Nalpha-[(2S)-2-benzyl-3-(tert-butylsulfonyl)propanoyl]-N-[(1S,2R,3S)-1-(cyclohexylmethyl)-3-cyclopropyl-2,3-dihydroxypropyl]-L-histidinamide | 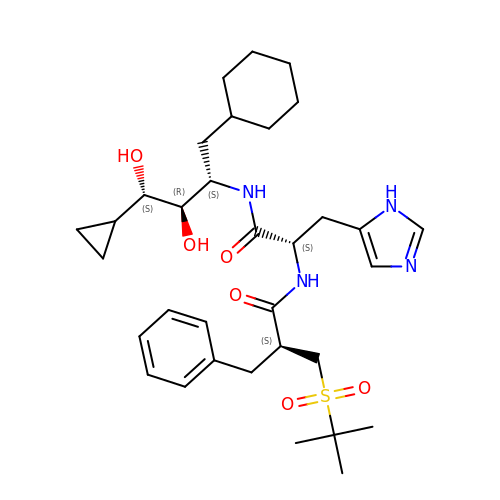C33 H50 N4 O6 S | UXIGZRQVLGFTOU-VQXQMPIVSA-N> GHMKKRKARSLLPLSTSLDHRSKEELHQDCLVLATAKHSRELNEDVSADVEERFHLGLFTDRATLYRMIDIEGKGHLENGHPELFHQLMLWKGDLKGVLQTAAERGELTDNLVAMAPAAGYHVWLWAVEAFAKQLCFQDQYVKAASHLLSIHKVYEAVELLKSNHFYREAIAIAKARLRPEDPVLKDLYLSWGTVLERDGHYAVAAKCYLGATCAYDAAKVLAKKGDAASLRTAAELAAIVGEDELSASLALRCAQELLLANNWVGAQEALQLHESLQGQRLVFCLLELLSRHLEEKQLSEGKSSSSYHTWNTGTEGPFVERVTAVWKSIFSLDTPEQYQEAFQKLQNIKYPSATNNTPAKQLLLHICHDLTLAVLSQQMASWDEAVQALLRAVVRSYDSGSFTIMQEVYSAFLPDGCDHLRDKLGDHQSPATPAFKSLEAFFLYGRLYEFWWSLSRPCPNSSVWVRAGHRTLSVEPSQQLDTASTEETDPETSQPEPNRPSELDLRLTEEGERMLSTFKELFSEKHASLQNSQRTVAEVQETLAEMIRQHQKSQLCKSTANGPDKNEPEVEAEQPLCSSQSQ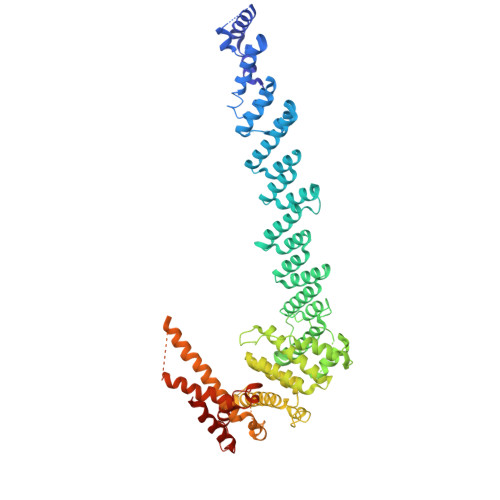CKEEKNEPLSLPELTKRLTEANQRMAKFPESIKAWPFPDVLECCLVLLLIRSHFPGCLAQEMQQQAQELLQKYGNTKTYRRHCQTFCM>[4x]MYDWFSEMRKKDPVYYDGNIWQVFSYRYTKEVLNNFSKFSSDLTGYHERLEDLRNGKIRFDIPTRYTMLTSDPPLHDELRSMSADIFSPQKLQTLETFIRETTRSLLDSIDPREDDIVKKLAVPLPIIVISK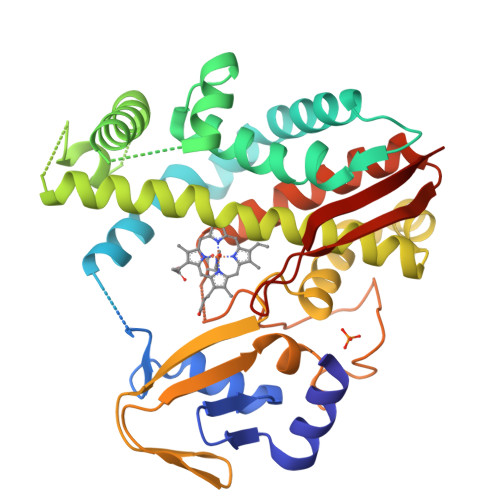ILGLPIEDKEKFKEWSDLVAFRLGKPGEIFELGKKYLELIGYVKDHLNSGTEVVSRVVNSNLSDIEKLGYIILLLIAGNEATTNLISNSVIDFTRFNLWQRIREENLYLKAIEEALRYSPPVMRTVRKTKERVKLGDQTIEEGEYVRVWIASANRDEEVFHDGEKFIPDRNPNPHLSFGSGIHLHLGAPLARLEARIAIEEFSKRFRHIEILDTEKVPNEVLNGYKRLVVRLKSNE6-ethyl-5-[(3~{S})-3-(6-pyridin-4-yl-1,3-benzodioxol-4-yl)but-1-ynyl]pyrimidine-2,4-diamine 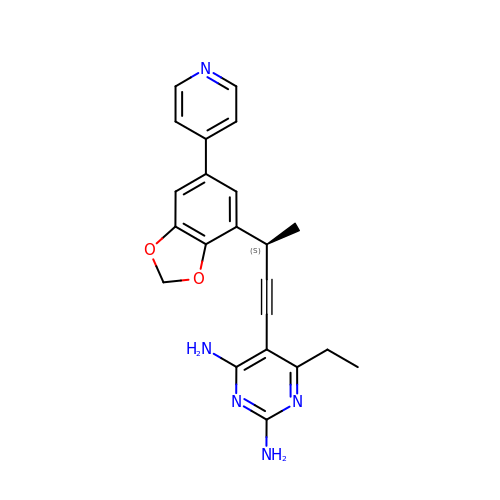| C22 H21 N5 O2 | NRVDPWMGAWNSHR-ZDUSSCGKSA-N> MEKTIKDTRKITEAMRLVAAAKVAAAQEQVMASRPFADRLAQVLYSLQTRLRFEDVDLPLLAKRPVKTVALLVVTGDRGLCGGYNTNVIRRAKERLQELEAEGLKYTLVIVGRKAAQYFQRRDYPIDAVYSGLEQIPSASEAGQIASELLSLFLSETVDRVELIYTKFVSLISSKPVVQTLLPLDPQGLETADDEIFRLTTRGSHLEVNREKVTSTLPALPSDMIFEQDPLQILDALLPLYLNNQLLRALQEAAASELAARMTAMNNASDNAQALILVP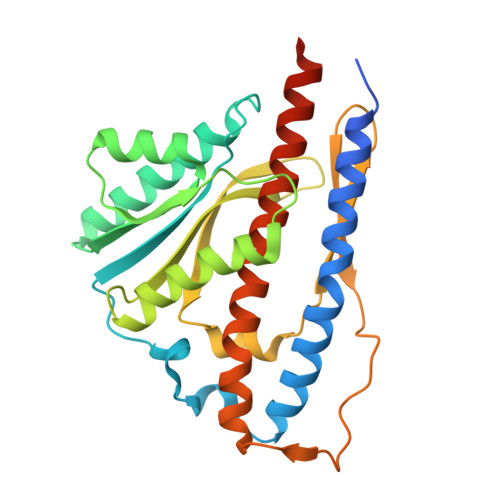R>[2x]MALVKIVRIETFPLFHRLEKPYGDANGFKRYRTCYLIRIITESGIDGWGECVDWLPALHVGFTKRIIPFLLGKQAGSRLSLVRTIQKWHQRAASAVSMALTEIAAKAADCSVCELWGGRYREEIPVYASFQSYSDSPQWISRSVSNVEAQLKKGFEQIKVKIGGTSFKEDVRHINALQHTAGSSITMILDANQSYDAAAAFKWERYFSEWTNIGWLEEPLPFDQPQDYAMLRSRLSV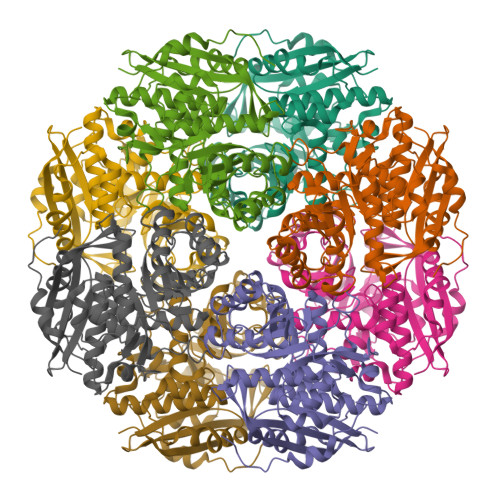PVAGGENMKGPAQYVPLLSQRCLDIIQPDVMHVNGIDEFRDCLQLARYFGVRASAHAYDGSLSRLYALFAQACLPPWSKMKNDHIEPIEWDVMENPFTDLVSLQPSKGMVHIPKGKGIGTEINMEIVNRYKWDGSAYEGHHHHHH>[2x]GMAPPSVFAEVPQAQPVLVFKLIADFREDPDPRKVNLGVGAYRTDDCQPWVLPVVRKVEQRIANNSSLNHEYLPILGLAEFRTCASRLALGDDSPALQEKRVGGVQSLGGTGALRIGAEFLARWYNGTNNKDTPVYVSSPTWENLNGVFTTAGFKDIRSYRYWDTEKRGLDLQGFLSDLENAPEFSIFVLLACAHNPTGTDPTPEQWKQIASVMKRRF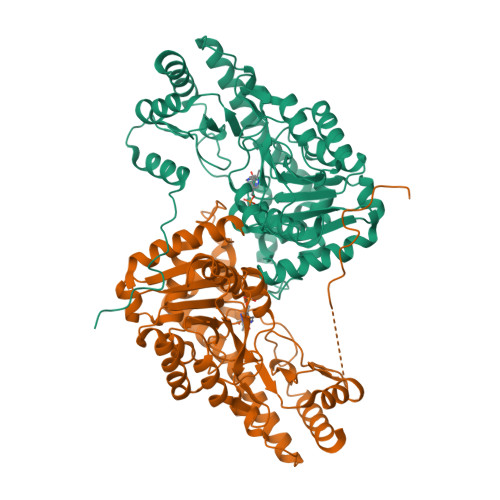LFPFFDSAYQGFASGNLEKDAWAIRYFVSEGFELFCAQSFSKNFGLYNERVGNLTVVAKEPDSILRVLSQMQKIVRVTWSNPPAQGARIVARTLSDPELFHEWTGNVKTMADRILSMRSELRARLEALKTPGTWNHITDQIGMFSFTGLNPKQVEYLINQKHIYLLPSGRINMCGLTTKNLDYVATSIHEAVTKIQ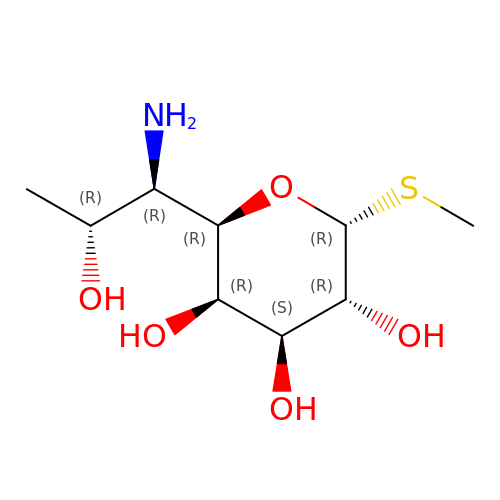(2R,3R,4S,5R,6R)-2-[(1R,2R)-1-azanyl-2-oxidanyl-propyl]-6-methylsulfanyl-oxane-3,4,5-triol | C9 H19 N O5 S | AEEIMWYSDWZKAT-HJTGYUAHSA-N> QEEGEDNGGEDNKKLRGALSSAILSEKPNVKWEDVAGLEGAKEALKEAVILPVKFPHLFKGNRKPTSGILLYGPPGTGKSYLAKAVATEANSTFFSVSSSDLVSKWMGESEKLVKQLFAMARENKPSIIFIDEVDALTGTRGEGESEASRRIKTELLVQMNGVGN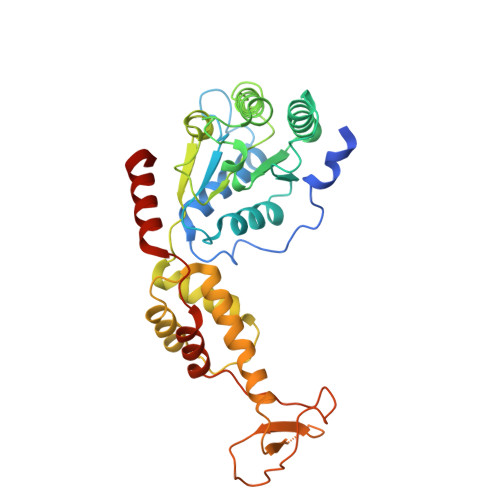DSQGVLVLGATNIPWQLDSAIRRRFERRIYIPLPDLAARTTMFEINVGDTPCVLTKEDYRTLGAMTEGYSGSDIAVVVKDALMQPIRKIQSATHFKDVSTEDDETRKLTPCSPGDDGAIEMSWTDIEADELKEPDLTIKDFLKAIKSTRPTVNEDDLLKQEQFTRDFGQEGN>[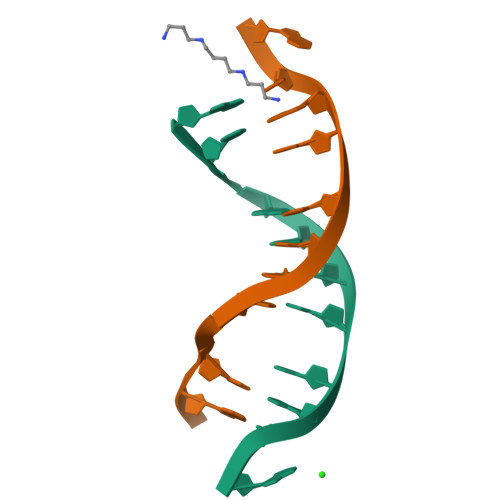2x]CGCNAATTXGCG>[2x]MDYRQLHRWDLPPEEAIKVQNELRKKIKLTPYEGEPE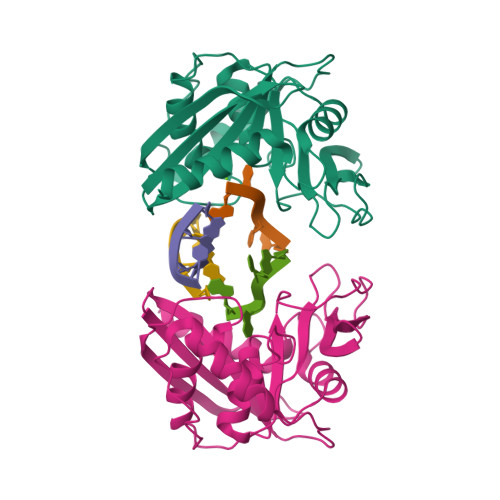YVAGVDLSFPGKEEGLAVIVVLEYPSFKILEVVSERGEITFPYIPGLLAFREGPLFLKAWEKLRTKPDVVVFDGQGLAHPRKLGIASHMGLFIEIPTIGVAKSRLYGTFKMPEDKRCSWSYLYDGEEIIGCVIRTKEGSAPIFVSPGHLMDVESSKRLIKAFTLPGRRIPEPTRLAHIYTQRLKKGLF> KETAAAKFERQHMDSSTSAASSSNYCNQMMKSRNLTKDRCKPVNTFVHESLADVQAVCSQKNVACKNGQTNCYQSYSTMSITD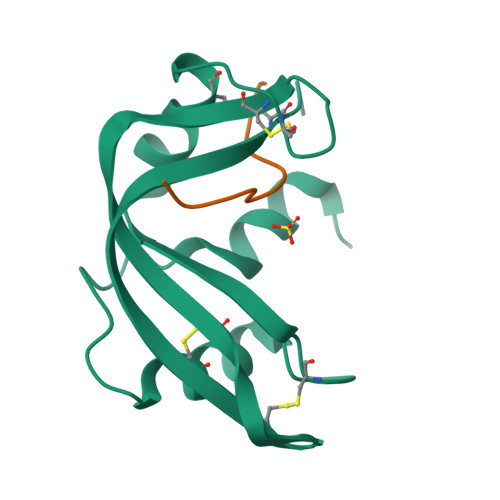CRETGSSKYPNCAYKTTQANKHIIVACEGN;> PYVPVHFAASV>QGPGGGGSVTCPGGQSTSNSQCCVWFDVLDDLQTNFYQGSKCESPVRKILRIVFHDAIGFS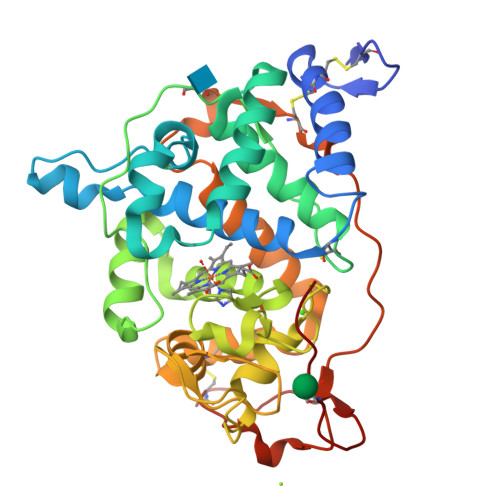PALTAAGQFGGGGADGSIIAHSNIELAFPANGGLTDTVEALRAVGINHGVSFGDLIQFATAVGMSNCPGSPRLEFLTGRSNSSQPSPPSLIPGPGNTVTAILDRMGDAGFSPDEVVDLLAAHSLASQEGLNSAIFRSPLDSTPQVFDTQFYIETLLKGTTQPGPSLGFAEELSPFPGEFRMRSDALLARDSRTACRWQSMTSSNEVMGQRYRAAMAKMSVLGFDRNALTDCSDVIPSAVSNNAAPVIPGGLTVDDIEVSCPSEPFPEIATASGPLPSLAPAP[2x]> VKVDEITDTTAQLSWTEGTDSHSPVISYAVQARTPFSVGWQSVRTVPEVIDGKTHTATVVEL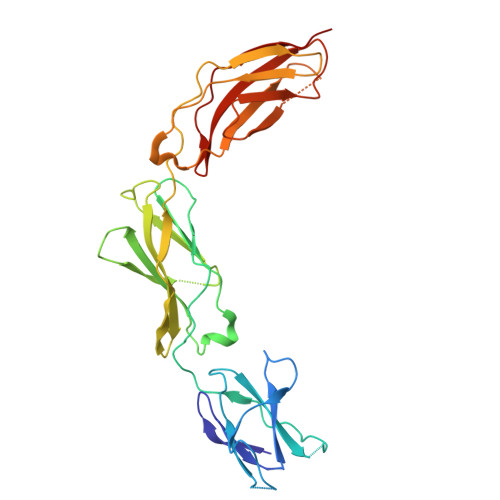NPWVEYEFRIVASNKIGGGEPSLPSEKVRTEEAAPEIAPSEVSGGGGSRSELVITWDPVPEELQNGGGFGYVVAFRPLGVTTWIQTVVTSPDNPRYVFRNESIVPFSPYEVKVGVYNNKGEGPFSPVTTVFSAEEEPTVAPSHISAHSLSSSEIEVSWNTIPWKLSNGHLLGYEVRYWNNGGEEESSRKVKVAGNQTSAVLRGLKSNLAYYTAVRAYNSAGAGPFSATVNATTKK1-[3-(trifluoromethyl)pyridin-2-yl]piperazine | C10 H12 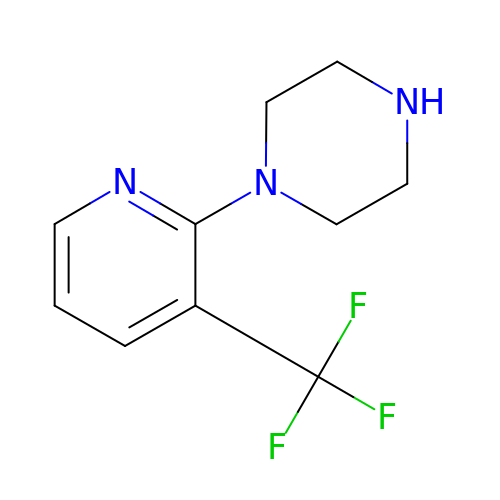F3 N3 | FRFKCMNQNNNZNO-UHFFFAOYSA-N> MGAPATVTEQGEDITSKKDRGVLKIVKRVGNGEETPMIGDKVYVHYKGKLSNGKKFDSSHDRNEPFVFSLGKGQVIKAWDI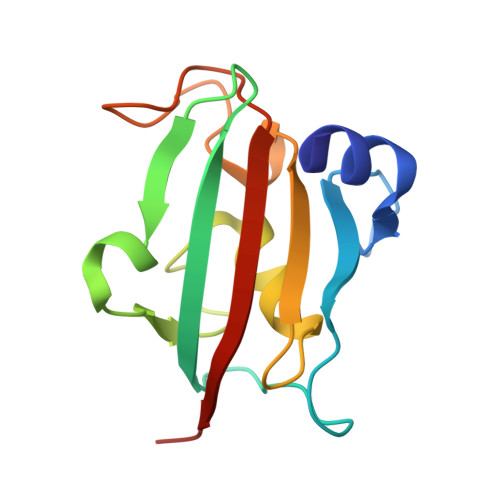GVATMKKGEICHLLCKPEYAYGSAGSLPKIPSNATLFFEIELLDFKGE> GHMTQSQTVTVDQQEILNRANEVEAPMADPPTDVPITPCELTAAKNAAQQLVLSADNMREYLAAGAKERQRLATSLRNAAKAYGEVDEEAATALDNDGEGTVQAESAGAVGGDSSAELTDTPRVATAGEPNFMDLKEAARKLETGDQGASLAHFADGWNTFNLTLQGDVKRFRGFDNWEGDAATACEASLDQQRQWILHMAKLSAAMAKQAQYVAQLHVWARREHPTYEDIVG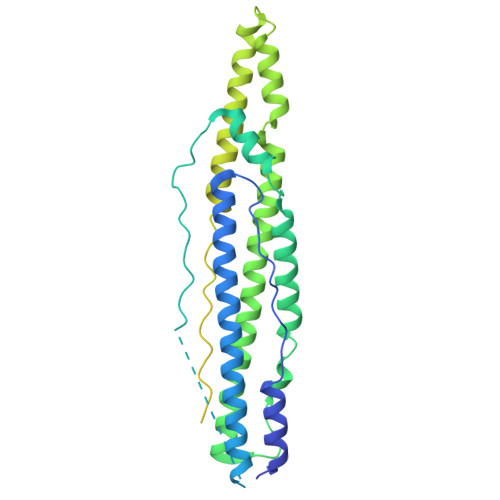LERLYAENPSARDQILPVYAEYQQRSEKVLTEYNNKAALEPVNPPKPPPAIKIDPPPPPQEQGLIPGFLMPPSDGSGVTPGTGMPAAPMVPPTGSPGGGLPADTAAQLTSAGREAAALSGDVAVKAASLGGGGGGGVPSAPLGSAIGGAESVRPAGAGDIAGLGQGRAGGGAALGGGGMGMPMGAAHQGQGGAKSKGSQQEDEALYTEDRAWTEAVIGNRRRQDSKESK>MSQPSTANGGFPSVVVTAVTATTSISPDIESTWKGLLAGESGIHALEDEFVTKWDLAVKIGGHLKD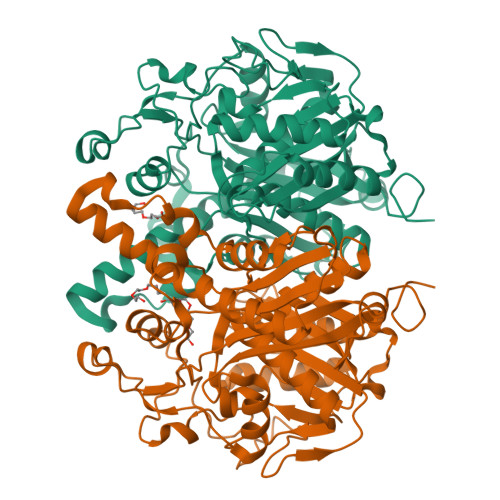PVDSHMGRLDMRRMSYVQRMGKLLGGQLWESAGSPEVDPDRFAVVVGTGLGGAERIVESYDLMNAGGPRKVSPLAVQMIMPNGAAAVIGLQLGARAGVMTPVSAQSSGSEAIAHAWRQIVMGDADVAVCGGVEGPIEALPIAAFSMMRAMSTRNDEPERASRPFDKDRDGFVFGEAGALMLIETEEHAKARGAKPLARLLGAGITSDAFHMVAPAADGVRAGRAMTRSLELAGLSPADIDHVNAHGTATPIGDAAEANAIRVAGCDQAAVYAPKSALGHSIGAVGALESVLTVLTLRDGVIPPTLNYETPDPEIDLDVVAGEPRYGDYRYAVNNSFGFGGHNVALAFGRY[8x]> MGSSHHHHHHSQDPENLYFQGDEITKKYIKDNIINVDDNIIKKKDIFKLKNENNEITECAFEYFESKKKFDDDIESRFFIINDNNYNENINLIYKDIKYCGLNIQTTGLEVFDENIRLIQIAVENYPVIIYDMFNINKKDILDGLRKVLENKNIIKIIQNGKFDAKFLLHNNFKIENIFDTYIASKLLDK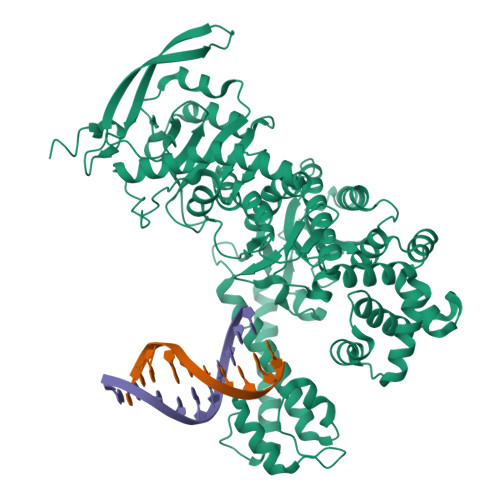NKNMYGFKLNNIVEKYLNVILDKQQQNSVWNNSLLNNNQLFYAARDSSCLLKLYKKLKEEIKKENLHIVNDIENKCILPICDMELNGIKVDLENLQKSTNEILNELNIEKDNLKKKLKDENINVNSQQQVLKALQKNNVRDISNKLIENTSDSNLKNFLNHEEIISLRNYRRLYKLYSAFYLKLPLHINTKTNKIHTTFNQLKTFSGRFSSEKPNLQQIPRQKNIREIFIPNDNNIFIIADFKQIELKIAAEITNDEIMLKAYNNNIDLHTLTASIITKKNIPDINKEDRHIAKAINFGLIYGMNYVNLKNYANTYYGLNMSLDQCLYFYNSFFEHYKGIYKWHNQVKQKRALQYSTLSNRKVIFPYFSFTKALNYPVQGTCADILKLALVDLYDNLKDINGKIILCVHDEIIIEVNKKFQEEALKILVQSMENSASYFLKKVKCEVSVKIAENWGSKD The Notch signalling pathway is highly conserved and plays key roles in many aspects of development and homeostasis. Canonical Notch signalling involves a simple cascade, whereby ligand binding induces successive cleavages to release the Notch intracellular domain (NICD) which translocates to the nucleus and directly regulates gene expression with its binding partners (Kovall, 2008; Kovall & Blacklow, 2010; Bray, 2016; Kovall et al, 2017). All Notch ligands have a similar architecture, with an extracellular domain consisting of multiple (7, 8, or 16) epidermal growth factor (EGF) repeats, a so‐called Delta/Serrate/Lag‐2 (DSL) domain and a highly conserved N‐terminal region (Bray, 2006; D’Souza et al, 2008; Kopan & Ilagan, 2009; Kovall & Blacklow, 2010). Receptor binding involves the N‐terminal portion including the DSL and N‐terminal domains (Cordle et al, 2008; Luca et al, 2015, 2017).

To determine whether the Drosophila ligands adopt the same arrangement as their mammalian counterparts, we solved the structures of the N‐terminal region of Drosophila Delta and Serrate as well as the ligand‐binding region of Drosophila Notch (EGF11‐13; Fig EV1A–E). Notable exceptions to the overall conserved arrangements are the β1‐2 and β5‐6 loops which exhibit different lengths and folding in the ligands. B–E The crystallographic asymmetric units are shown for the three structures (B) Delta—one copy of C2‐DSL‐EGF1 construct; (C) Serrate—two copies of C2‐DSL‐EGF1‐EGF2 construct; (D) C2 domain of Drosophila Delta (rainbow colouring) overlaid on the same region of Drosophila Serrate (grey). Disulphide bonds are shown as yellow sticks and the bound calcium ion in the Serrate structure as a grey sphere. The β1‐2 loop (blue for Delta, at top) adopts a different conformation in Delta than in Serrate despite conservation of the two stabilizing disulphides; (E) Notch—one copy of EGF11‐13. Likewise, the equivalent fragment containing SerrateΔβ1‐2 loop deletion (removal of residues LRATK) also exhibited reduced binding to liposomes, although to a variable extent that was not reproducibly significant. This may be due to differences in the lipid‐binding specificities because we have previously noted the heterogeneity of the C2 loop sequences in different ligand families and hypothesized that they may confer different lipid‐binding specificities (Suckling et al, 2017). Combining SerΔβ1‐2 allele with this double‐mutant chromosome enhanced the thickening of veins in a similar manner to DlΔβ1‐2 (Fig EV2C and D).

>AGNFELEILEISNTNSHLLNGYCCGMPAELRATKTIGCSPCTTAFRLCLKEYQTTEQGASISTGCSFGNATTKILGGSSFVLSDPGVGAIVLPFTFRWTKSFTLILQALDMYNTSYPDAERLIEETSYSGVILPSPEWKTLDHIGRNARITYRVRVQCAVTYYNTTCTTFCRPRDDQFGHYACGSEGQKLCLNGWQGVNCEEAICKAGCDPVHGKCDRPGECECRPGWRGPLCNECMVYPGCKHGSCNGSAWKCVCDTNWGGILCDQDLN[2x]> GAADKGEIRVGNRYQADITDLLKEGEEDGRDQSRLETQVWEAHNPLTDKQIDQFLVVARSVGTFARALDCSSSVRQPSLHMSAAAASRDITLFHAMDTLHKNIYDISKAISALVPQGGPVLCRDEMEEWSASEANLFEEALEKYGKDFTDIQQDFLPWKSLTSIIEYYYMWKTTDRYVQQKRLKAAEAESKLKQV;> MAQTQGTRRKVCYY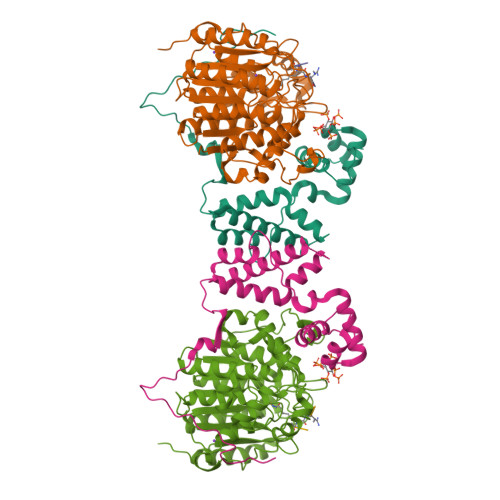YDGDVGNYYYGQGHPMKPHRIRMTHNLLLNYGLYRKMEIYRPHKANAEEMTKYHSDDYIKFLRSIRPDNMSEYSKQMQRFNVGEDCPVFDGLFEFCQLSTGGSVASAVKLNKQQTDIAVNWAGGLHHAKKSEASGFCYVNDIVLAILELLKYHQRVLYIDIDIHHGDGVEEAFYTTDRVMTVSFHKYGEYFPGTGDLRDIGAGKGKYYAVNYPLRDGIDDESYEAIFKPVMSKVMEMFQPSAVVLQCGSDSLSGDRLGCFNLTIKGHAKCVEFVKSFNLPMLMLGGGGYTIRNVARCWTYETAVALDTEIPNELPYNDYFEYFGPDFKLHISPSNMTNQNTNEYLEKIKQRLFENLRMLPHA;> LGKGGAXRH> PISPIETVPVKLKPGMDGPKVKQWPLTEEKIKALVEICTELEKEGKISKIGPENPYNTPVFAIKKKDSTKWRKLVDFRELNKRTQDFWEVQLGIPHPAGLKKKKSVTVLDVGDAYFSVPLDEDFRKYTAFTIPSINNETPGIRYQYNVLPQGWKGSPAIFQSSMTKILEPFRKQNPDIVIYQY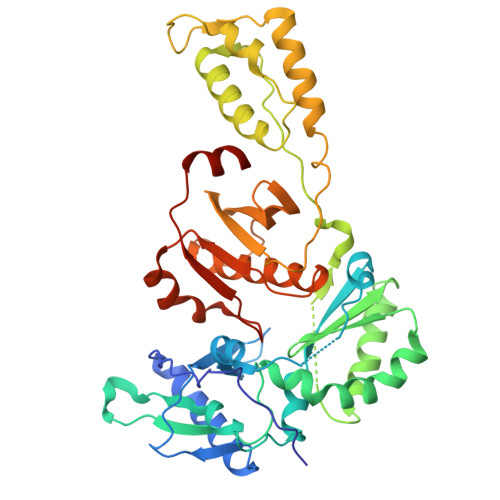MDDLYVGSDLEIGQHRTKIEELRQHLLRWGLYTPDKKHQKEPPFLWMGYELHPDKWTVQPIVLPEKDSWTVNDIQKLVGKLNWASQIYPGIKVRQLCKLLRGTKALTEVIPLTEEAELELAENREILKEPVHGVYYDPSKDLIAEIQKQGQGQWTYQIYQEPFKNLKTGKYARMRGAHTNDVKQLTEAVQKITTESIVIWGKTPKFKLPIQKETWETWWTEYWQATWIPEWEFVNTPPLVKLWYQLEKEPIVGAETF> GVDYKYKQKPKYQVRWKIIESYEGNSYTFIDPTQLPYNEKWEFPRNNLQFGKTLGAGAFGKVVEATAFGLGKEDAVLKVAVKMLKSTAHADEKEALMSELKIMSHLGQHENIVNLLGACTHGGPVLVITEYCCYGDLLNFLRRKRPPGLEYSYNPSHNPEEQLSSRDLLHFSSQVAQGMAFLASKNCIHRDVAARNVLLTNGHVAKIGDFGLARDIMNDSNYIVKGNARLPVKWMAPESIFDCVYTVQSDVWSYGILLWEIFSLGLNPYPGILVNSKFYKLVKDGYQMAQPAFAPKNIYSIM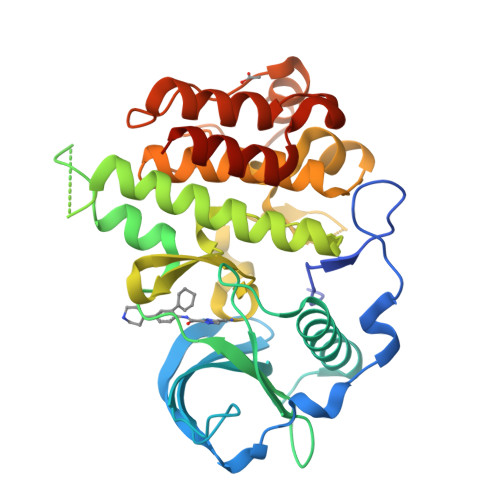QACWALEPTHRPTFQQICSFLQEQAQEDRRERD N-{(2R,4S,5S)-2-benzyl-5-[(tert-butoxycarbonyl)amino]-4-hydroxy-6-phenylhexanoyl}-L-leucyl-L-phenylalaninamide | C39 H52 N4 O6 | 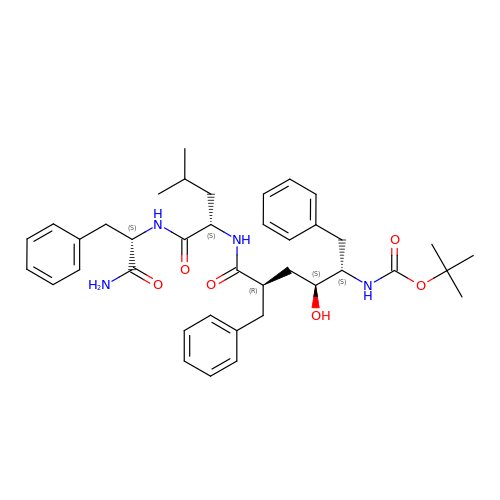MURCDOXDAHPNRQ-OWIQAHIBSA-N>AMIYGIG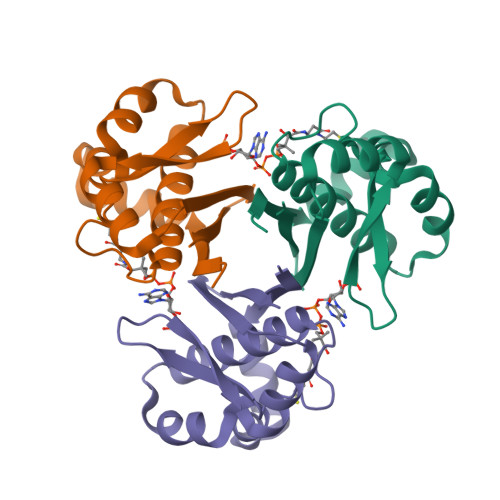TDIVSLKRIIRLNKKFGQAFAGRILTPEELLEFPQAGKPVNYLAKRFAAKEAFAKAVGTGIRGAVSFRNIGIGHDALGKPEFFYGPALSKWLEEQGISRVSLSMSDEEDTVLAFVVAEK[3x]>RSSHHHHHHGEFDIPTTENLYFQSGIRRKCPNVLNDPVNVRINCIPEQFPTEGICAQRGCCWRPWNDSLIPWCFFVDNHGYNVQDMTTTSIGVEAKLNRIPSPTLFGNDINSVLFTTQNQTPNRFRFKITDPNNRRYEVPHQYVKEFTGPTVSDTLYDVKVAQNPFSIQVIRKSNGKTLFDTSIGPLVYSDQYLQISARLPSDYIYGIGEQVHKRFRHDLSWKTWPIFTRDQLPGDNNNNLYGHQTFFMCIEDTSGKSFGVFLMNSNAMEIFIQPTPIVTYRVTGGILDFYILLGDTPEQVVQQYQQLVGLPAMPAYWNLGFQLSRWNYKSLDVVKEVVRRNREAGIPFDTQVTDIDYMEDKKDFTYDQVAFNGLPQFVQDLHDHGQKYVIILDPAISIGRRANGTTYATYERGNTQHVWINESDGSTPIIGEVWPGLTVYPDFTNPNCIDWWANECSIFHQEVQYDGLWIDMNEVSSFIQGSTKGCNVNKLNYPPFTPDILDKLMYSKTICMDAVQNWGKQYDVHSLYGYSMAIATEQAVQKVFPNKRSFILTRSTFAGSGRHAAHWLGDNTASWEQMEWSITGMLEFSLFGIPLVGADICGFVAETTEELCRRWMQLGAFYPFSRNHNSDGYEHQDPAFFGQNSLLVKSSRQYLTIRYTLLPFLYTLFYKAHVFGETVARPVLHEFYEDTNSWIEDTEFLWGPALLITPVLKQGADTVSAYIPDAIWYDYESGAKRPWRKQRVDMYLPADKIGLHLRGGYIIPIQEPDVTTTASRKNPLGLIVALGENNTAKGDFFWDDGETK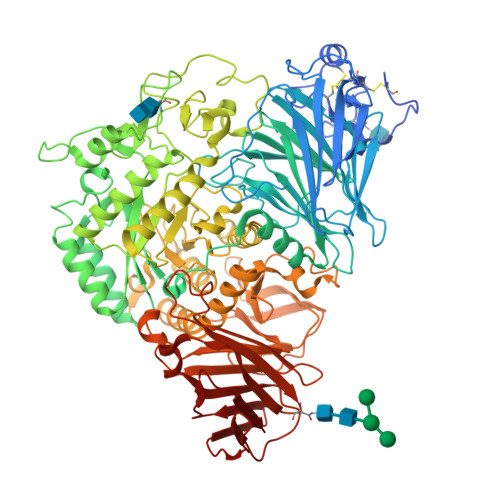DTIQNGNYILYTFSVSNNTLDIVCTHSSYQEGTTLAFQTVKILGLTDSVTEVRVAENNQPMNAHSNFTYDASNQVLLIADLKLNLGRNFSVQW[4x]>[2x]AKPLTDQEKRRQISIRGIVGVENVAELKKSFNRHLHFTLVKDRNVATTRDYYFALAHTVRDHLVGRWIRTQQHYYDKCPKRVYYLSLEFYMGRTLQNTMINLGLQNACDEAIYQLGLDIEELEEIEE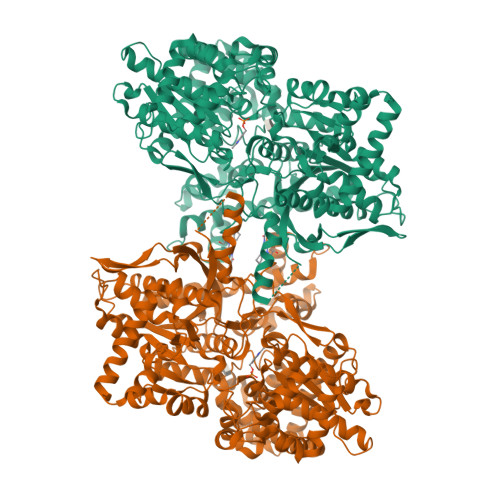DAGLGNGGLGRLAACFLDSMATLGLAAYGYGIRYEYGIFNQKIRDGWQVEEADDWLRYGNPWEKSRPEFMLPVHFYGKVEHTNTGTKWIDTQVVLALPYDTPVPGYMNNTVNTMRLWSARAPNDFNLRDFNVGDYIQAVLDRNLAENISRVLYPNDNFFEGKELRLKQEYFVVAATLQDIIRRFKASKFGSTRGAATVFDAFPDQVAIQLNDTHPALAIPELMRIFVDIEKLPWSKAWELTQKTFAYTNHTVLPEALERWPVDLVEKLLPRHLEIIYEINQKHLDRIVALFPKDVDRLRRMSLIEEEGSKRINMAHLCIVGSHAVNGVAKIHSDIVKTKVFKDFSELEPDKFQNKTNGITPRRWLLLCNPGLAELIAEKIGEDYVKDLSQLTKLHSFLGDDVFLRELAKVKQENKLKFSQFLETEYKVKINPSSMFDVQVKRIHEYKRQLLNCLHVITMYNRIKKDPKKLFVPRTVIIGGKAAPGYHMAKMIIKLITSVADVVNNDPMVGSKLKVIFLENYRVSLAEKVIPATDLSEQISTAGTEASGTGNMKFMLNGALTIGTMDGANVEMAEEAGEENLFIFGMRIDDVAALDKKGYEAKEYYEALPELKLVIDQIDNGFFSPKQPDLFKDIINMLFYHDRFKVFADYEAYVKCQDKVSQLYMNPKAWNTMVLKNIAASGKFSSDRTIKEYAQNIWNVEPSDLKISLSNESNKVNGN5,10-DIMETHYLENE TETRAHYDROMETHANOPTERIN | C31 H45 N6 O16 P | 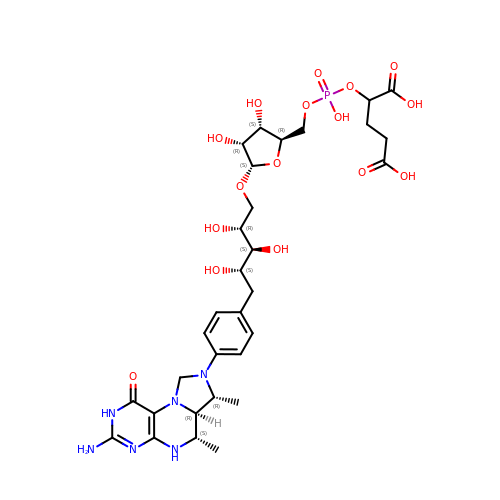GBMIGEWJAPFSQI-UQXKJNEMSA-N> CUCTUCTTC;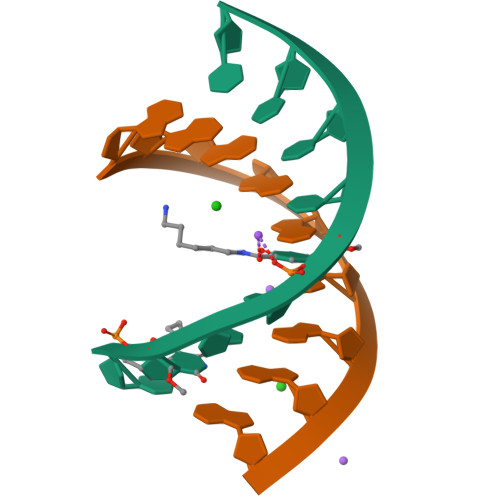> GAAGAAGAG> GLGDELEEVIVEKTKQTVASISSGPKHTQKVPILTANETGAT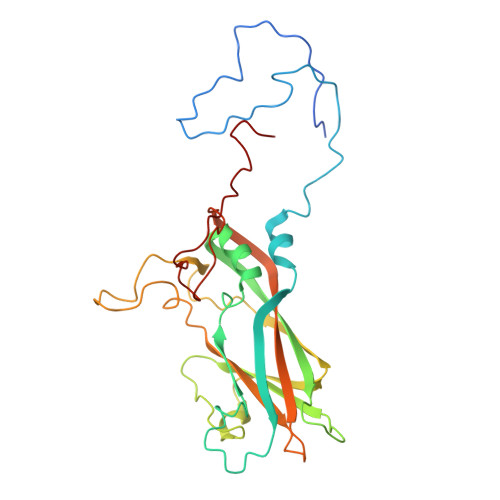MPVLPSDSIETRTTYMHFNGSETDVECFLGRAACVHVTEIQNKDATGIDNHREAKLFNDWKISLSSLVQLRKKLELFTYVRFDSEYTILATASQPDSANYSSNLVVQAMYVPPGAPNPKEWDDYTWQSASNPSVFFKVGDTSRFSVPYVGLASAYNCFYDGYSHDDAETQYGITVLNHMGSMAFRIVNEHDEHKTLVKIRVYHRAKHVEAWIPRAPRALPYTSIGRTNYPKNTEPVIKKRKGDIKSY>MAKAHIELTINGHPVEALVEPRTLLIHFIREQQNLTGAHIGCDTSHCGACTVDLDGMSVKSCTMFAVQANGASITTIEGMAAPDGTLSALQEGFRMMHGLQCGYCTPGMIMRSHRLLQENPSPTEAEIRFGIGGNLCRCTGYQNIVKAIQYAAAKINGVPFEEAAE[2x];>MNIQTTVEPTSAERAEKLQGMGCKRKRVEDIRFTQGKGNYVDDVKLPGMLFGDFVRSSHAHARIKSIDTSKAKALPGVFAVLTAADLKPLNLHYMPTLAGDVQAVLADEKVLFQNQEVAFVVAKDRYVAADAIELVEVDYEPLPVLVDPFKAMEPDAPLLREDIKDKMTGAHGARKHHNHIFRWEIGDKEGTDATFAKAEVVSKDMFTYHRVHPSPLETCQCVASMDKIKGELTLWGTFQAPHVIRTVVSLISGLPEHKIHVIAPDIGGGFGNKVGAYSGYVCAVVASIVLGVPVKWVEDRMENLSTTSFARDYHMTTELAATKDGKILAMRCHVLADHGAFDACADPSKWPAGFMNICTGSYDMPVAHLAVDGVYTNKASGGVAYRCSFRVTEAVYAIERAIETLAQRLEMDSADLRIKNFIQPEQFPYMAPLGWEYDSGNYPLAMKKAMDTVGYHQLRAEQKAKQEAFKRGETREIMGIGISFFTEIVGAGPSKNCDILGVSMFDSAEIRIHPTGSVIARMGTKSQGQGHETTYAQIIATELGIPADDIMIEEGNTDTAPYGLGTYGSRSTPTAGAATAVAARKIKAKAQMIAAHMLEVHEGDLEWDVDRFRVKGLPEKFKTMKELAWASYNSPPPNLEPGLEAVNYYDPPNMTYPFGAYFCIMDIDVDTGVAKTRRFYALDDCGTRINPMIIEGQVHGGLTEAFAVAMGQEIRYDEQGNVLGASFMDFFLPTAVETPKWETDYTVTPSPHHPIGAKGVGESPHVGGVPCF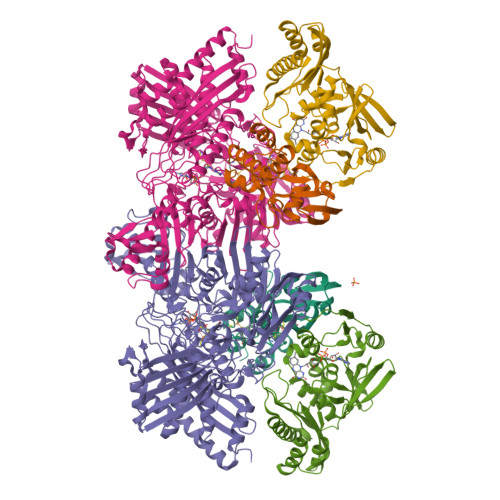SNAVNDAYAFLNAGHIQMPHDAWRLWKVGEQLGLHV[2x];>[2x]MIPGSFDYHRPKSIADAVALLTKLGEDARPLAGGHSLIPIMKTRLATPEHLVDLRDIGDLVGIREEGTDVVIGAMTTQHALIGSDFLAAKLPIIRETSLLIADPQIRYMGTIGGNAANGDPGNDMPALMQCLGAAYELTGPEGARIVAARDYYQGAYFTAIEPGELLTAIRIPVPPTGHGYAYEKLKRKIGDYATAAAAVVLTMSGGKCVTASIGLTNVANTPLWAEEAGKVLVGTALDKPALDKAVALAEAITAPASDGRGPAEYRTKMAGVMLRRAVERAKARAKN> AATAPAGASTTSSTSSAQKSFFKTTEMIGYVHSIDGTIATLIPAPGNPGVAYNTIIQIQVSPTTFAAGLVFNLEKDGRIGIILMDNI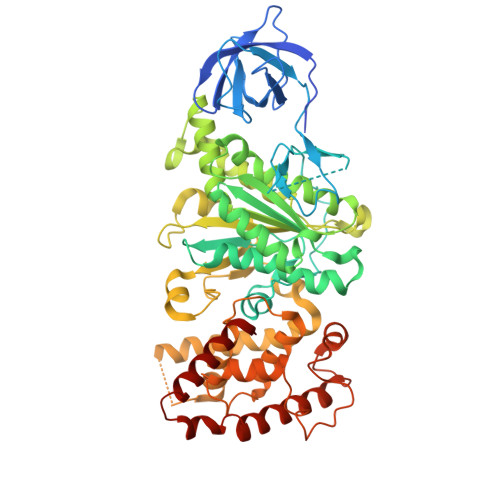TEVQSGQKVMATGQLLHIPVGAGVLGKVVNPLGHEVPVGLVTRSRRLLDSTLGKVDTGAPNIVSRSPVNYNLLTGFKAVDTMIPIGRGQRELIVGDRQTGKTSIAVSTIINQVRINQQILSKNAVISIYVSIGQRCSNVARIHRLLQSYGALRYTTVMAATAAEPAGLQYLAPYAGVTMGEYFMNRGRHCLCVYDDLSKQAVAYRQISLLLRRPPGREAYPGDVFYLHSRLLERAAMLSPGKGGGSVTALPIVETLSNDVTAYIVTNVISITDGQIYLDTKLFTGGQRPAVNIGLSVSRVGSSAQNAAMKGVAGKLKGILAEYRKLAADSVGGQQVQTIPMIRGARFVALFNQKQPSYFMNAIVSLYACLNGYLDDVKVQYVKFYEYLLVHRDLGIMYGTAKNKFFYMYVQELNYLIRFFTLNSPILHGELEEMLKQHTHLFLQHYQSKMNAIKSEKDVKALKNLLYSCKRAV> DFSIV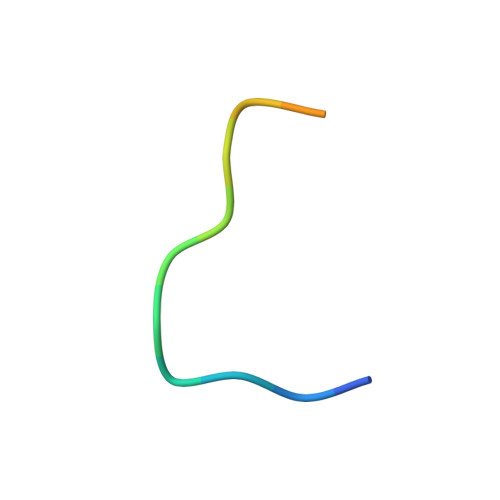GSLPRDFELS> YDPDQYSIEADKKFKYSVKLSDYPTLQDAASAAVDGLLIDRDYNFYGGETVDFGGKVLTIECKAKFIGDGNLIFTKLGKGSRIAGVFMESTTTPWVIKPWTDDNQWLTDAAAVVATLKQSKTDGYQPTVSDYVKFPGIETLLPPNAKGQNITSTLEIRECIGVEVHRASGLMAGFLFRGCHFCKMVDANNPSGGKDGIITFENLSGDWGKGNYVIGGRTSYGSVSSAQFLRNNGGFERDGGVIGFTSYRAGGSGVKTWQGTVGSTTSRNYNLQFRDSVVIYPVWDGFDLGADTDMNPELDRPGDYPITQYPLHQLPLNHLIDNLLVRGALGVGFGMDGKGMYVSNITVEDCAGSGAYLLTHESVFTNIAIIDTNTKDFQANQIYISGACRVNGLRLIGIRSTDGQSLTIDAPNSTVSGITGMVDPSRINVANLAEEGLGNIRANSFGYDSAAIKLRIHKLSKTLDSGALYSHIN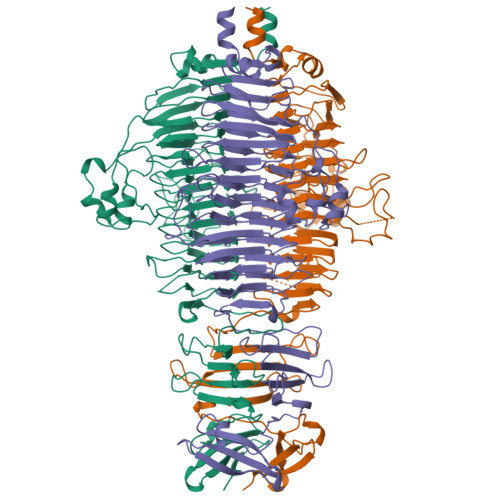GGAGSGSAYTQLTAISGSTPDAVSLKVNHKDCRGAEIPFVPDIASDDFIKDSSCFLPYWENNSTSLKALVKKPNGELVRLTLATL>ADLLVKTPEAYDQALKKAKPGDDIILANGTWRDFEVLFEAKGNENKPITLRGQTPGKVFLTGQSNLRLAGEHLIVSGLVFKDGYTPTGEVIAFRRNKDVLASHSRVTQVVIDNFSNPEKFEQDSWVMVYGRHNRFDHNHLVGKRNKGVTMAVRLTTESSQQNHHRIDHNYFGPRPILGSNGGETLRIGTSHHSLTDSFTLVENNYFDRCNGEVEIISNKSGKNSIRNNVFFESRGTLTLRHGNGNIVENNVFFGNGVDHTGGIRVINRDQIIRNNYLEGLTGYRFGSGLTVMNGVPNSKINRYHQVDNALIENNTLVNVEHIQFAAGSDKERSAAPINSNMNNNLIVNDQGTDGITAFDDISGIKFKDNLLNQDAKPSINKGFEQADITMQRHDNGLLYPEAKTQQKYGVSTQLEPIGKDEVGVSWYPKVEPDVAFGSGKHIAVSPGDNTLFDAIASAETGDVLVLQAGEYWVSKILSLDKTLTIRAQEKGSAVIFPQRSTLIEINNKGNLTLDGVYVDATNAPDAAGNTLIRTTRLPMQRNYRLAIKNSTFENLDINHSYHFFDAGNRSFADYIEVQDSQFKHITGDLFRLNKETDDLGIYNVEYLTIENSNVSDLQGAIAKVYRGGTDESTFGPHVVMNNNIFNEVGKGKRNKSAASLILHGTQVNKMTTNEFNNSAPIIFEL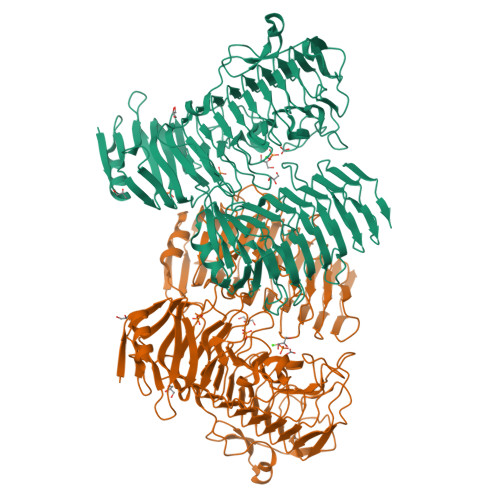TVGEPKTWVTGNVFEGTPEPVVRDLFPLSGATTTISGNTVL[4x]> MSKENALFPAVKDAIVFDALWQQAHEKVTALSGEIWTDTGDHDPGVTLLQSATWNCSDLSYRASLSLNDLLTHQDQSTLFPEEFGPEQVLTCNTVTAEDYRRALLDVHSSDIQALDTPEQDFLFSDVSLTQEPKEHRFHWWYNAEKREYSFRKPTDSGEVNELKLRGNLWLSLVPTRYTQSLSPENLAAVEQCLAEFLAAHRNLGEVVSRITWLQPATFSPRMTIELADNIGDINQVAAQIYQVTDAFLRPAVARYTTEQRRALGDADDAIFEGPRLKHGWQQTAPSQITSGGYVLNLGPLVNLLLAIPGVASLSTLSVDKGDGHITAVTGDNLRWQVADGYYPLLWGAPPLSLLAGDDSPLTLVSKGGIRNTLESEAMAGYLTQADLIVTTPTVLPAGRFRDQTLYIPIGQRQPECYALQQPDTVIDDQTRAVHQFLLPVDQLLADGTAELAQLPTLLAFKNRGDAIRGTRWPYTNAMVQQAIHQPYAKTLEAIAQQDAAIFTQDKQPVGGNYARELDFLQYLLGYFGTQRAALPLTLDLPDFLATQRAYLAQQPALGYDRINIRIDQVSALQKRIAARIGLDSICFADNPDLGQLPFYLIEHRQLLPQTPDSTFDSEQTPSGFAVAEPDITLTQAGSVGKVVQGQLIDLIAIEGGSRLHVSRLLVIKAEGDSFTVSTENSQQLHNTLSRLETAWASHNLRWQNSNVWLQDMDYRLNYAEAKLQPANPQQRLLASNAQSPYPAMVSVGDGIVLRPAGLQFYMPGANATRAATLDADWQLAATVKAVDPIAGTLLIEKAAGSTEDFPSAESSFRYQW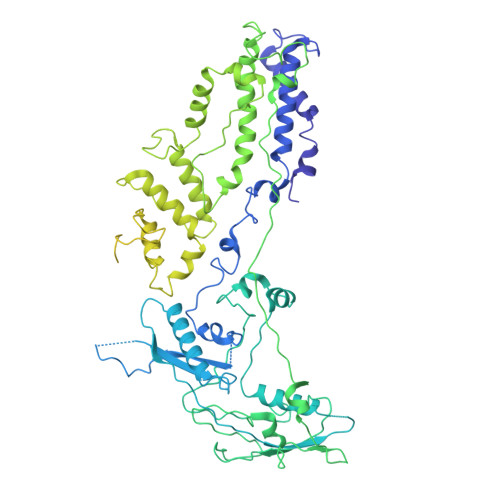AFSQANYATTDRFSFVVSAVLNRRLIENPNIVPEQLVAWIQETIMAEFPAHVSLINHWLDDATFNNFGVTYSRWQNSGMPLGDDAFALMQILTLGHLPVTQLDIGLMRIATEEQRTEVIGDGSQWHEDVILREELFYVPKDVQTTL GuaB catalyzes the oxidation of the substrate inosine-5´-monophosphate (IMP) to xanthosine 5´-monophosphate (XMP) using NAD+ as a cofactor, and guanosine 5´-monophosphate (GMP) synthase converts XMP to guanosine 5'- monophosphate (GMP) to generate guanine nucleotides essential for cell growth and viability. Indeed, genetic studies have shown that de novo guanine biosynthesis is essential for growth and viability of bacteria both in vitro and in vivo (10–23). Here, we present the first high resolution co-crystal structures of A. baumannii, S. aureus, and E. coli GuaB proteins (cystathionine beta-synthase (CBS) domains deleted), each determined with a matched set of three different inhibitors bound. Similarly, the NAD+ binding region, also where our compounds bind, occurs at the junction between neighboring molecules with side chains from both protomers contributing to ligand binding interactions.

The novel S. aureus and E. coli structures crystallize with one molecule in the asymmetric unit (asu), yet re-create the common GuaB tetramer arrangement via the fourfold symmetry operator of their I4 space group. We observed a tight overlay of structures across the bacterial strains, highlighting common critical interactions required for potency. These inhibitors mimic the NADH/IMP cofactor interactions by forming strong π-π stacking interactions with IMP while also hydrogen bonding with the conserved glycine (Gly299Ab/302Sa/300Ec) which is one of the two hydrogen bond interactions observed with the NADH amide. The ligand linker segment induces a 90° bend, directing either the amide N-H of G2 and G1 or the imidazole of G8 to form an important hydrogen bond to the conserved glutamic acid (Glu416Ab/417Sa/415Ec) while directing the aryl tail group into a hydrophobic shelf region. Differences in the polarity of a particular key selectivity residue specifically (Ser250 in E. coli versus Ala252 in S. aureus and Ala249 in A. baumannii) was found to be critical for inhibitor interaction with GuaB which corroborates the observations of previous reports. The key residues (SER-440 and SER-250) in the binding site of GuaB E. coli contribute to a stable and extensive water network (more green and well-connected spheres) predicted by WaterMap analysis with the pseudo-apo crystal structures. To disrupt such water network, the compound needs to pay a larger desolvation penalty leading to poor potency, whereas the same compound binding to GuaB in S. aureus and A. baumannii does not need to pay for such penalty with a less favorable water network (more red and less connected spheres). Based on our analysis of the water networks present in these structures, we hypothesize that differences in the free energy of solvation of the binding site produce the observed difference in binding activity.

> MHHHHHHGENLYFQGSLRIAKEALTFDDVLLVPAHSTVLPNTADLSTQLTKTIRLNIPMLSAAMDTVTEARLAIALAQEGGIGFIHKNMSIERQAEEVRRVKKHSGGLRVGAAVGAGAGNEERVDALVAAGVDVLLIDSSHGHSEGVLQRIRETRAKYPDLQIIGGNVATAAGARALAEAGCSAVKVGIGPGSICTTRIVTGVGVPQITAVADAVEALEGTGIPVIADGGIRFSGDIAKAIAAGASAVMVGSMLAGTEESPGEIELYQGRSYKSYRGMGSLGAMSKGSSDRYFQSDNAADKLVPEGIEGRVAYKGRLKEIIHQQMGGLRSCMGLTGCGTIDELRTKAEFVRISGAGIQESHVHDVTITKESPNYRLGSGNS>[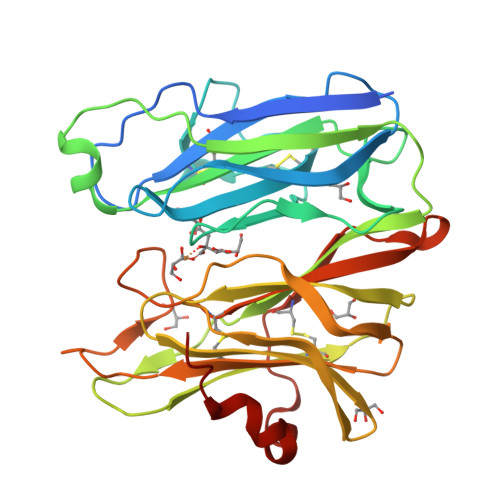2x]NECLGTIGPVTPLDASDFALDIRMPGVTPKESDTYFCMSMRLPVDEEAFVIDFKPRASMDTVHAMLLFGCNMPSSTGSYWFCDEGTCTDKANILYAWARNAPPTRLPKGVGFRVGGETGSKYFVLQVHYGDISAFRDNHKDCSGVSVHLTRVPQPLIAGMYLMMSVDTVIPPGEKVVNADISCQYKMYPMHVFAYRVHTHHLGKVVSGYRVRNGQWTLIGRQNPQLPQAFYPVEHPVDVTFGDILAARCVFTGEGRTEATHIGGTSSDEMCNLYIMYYMEAKYALSFMTCTKNVAPDMFRTIPAEANIPIPV>PVMHPHGVPPSHRPWQMKDLQAIKQEVSQAAPGSPQFMQTIRLAVQQFDPTAKDLQDLLQYLCSSLVASLHHQQLDSLISEAETRGITGYNPLAGPLRVQANNPQQQGLRREYQQLWLTAFAALPGSAKDPSWASILQGLEEPYHTFVERLNVALDNGLPEGTPKDPILRSLAYSNANKEC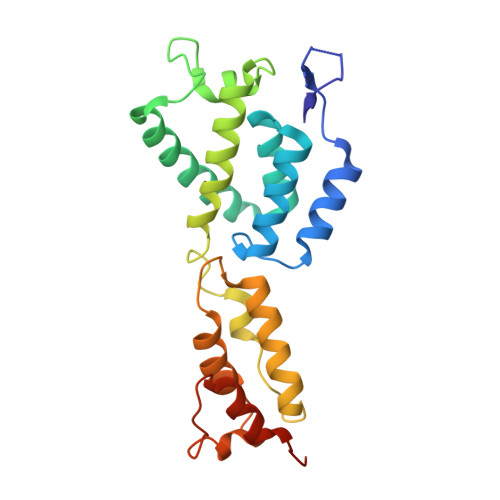QKLLQARGHTNSPLGDMLRACQAWTPKDKTKVL[3x]> GMNPEYDYLFKLLLIGDSGVGKSCLLLRFADDTYTDSYISTIGVDFKIRTISLENKTVKLQIWDTAGQERFRTITSSYYRGAHGIIIVYDVTDRDSFDNVKQW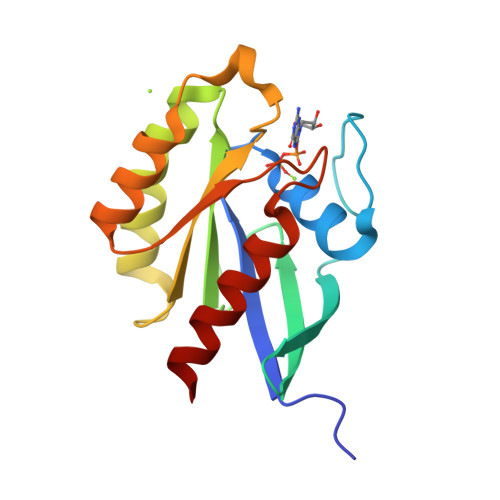IQEIDRYAMENVNKLLVGNKCDLVSKRVVTSDEGRELADSHGIKFIETSAKNAYNVEQAFHTMAGEIKKRVQ>[2x]MSSFSTQTPYPNLAVPFFTSIPNGLYPSKSIVISGVVLSDAKRFQINLRCGGDIAFHLNPRFDENAVVRNTQI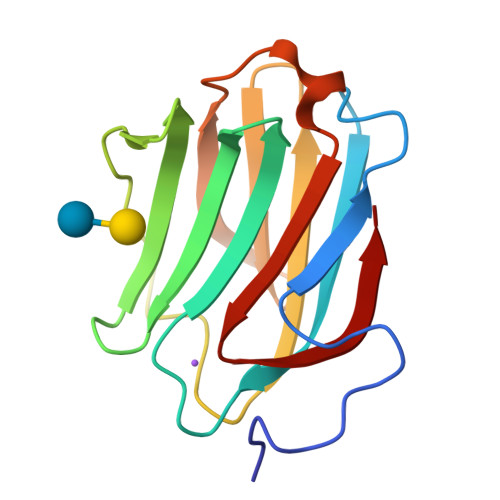NNSWGPEERSLPGSMPFSRGQRFSVWILCEGHCFKVAVDGQHICEYSHRLMNLPDINTLEVAGDIQLTHVET>KLATDIENNVRVVVYIRKDVEDNSQTIEKEGQTVTNNDYHKVYDSLKNMSTVKSVTFSSKEEQYEKLTEIMGDNW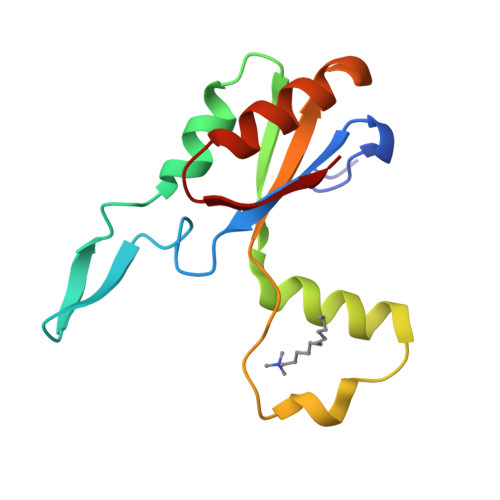KIFEGDANPLYDAYIVEANAPNDVKTIAEDAKKIEGVSEVQD[2x]>[2x]MKTDFIMVPTAMPDEKMINYQLAIDGGEPVIPKANRKTIFPNIAKEDLFQMMISVQKPEEMVVSEFAEKYRQRVGAPYAIPTASGTSSLHLALVGAGVKAGDEVIVPAFTFIATAQAIVAAKAIPVFADIDPQTYCLDPRQLDKKVTARTKAVMPVHVHGLPADIDALASFCRQHQLALIEDASHAHSATLHGRYCGTFGDAAGQSLMADKNFPLGGEAGIAFFKERESYDRALAFLEESGLDYRMSWVAAAFGISQLDRLDYYDEIRQRNAQRLIDELATTRLFTGPMI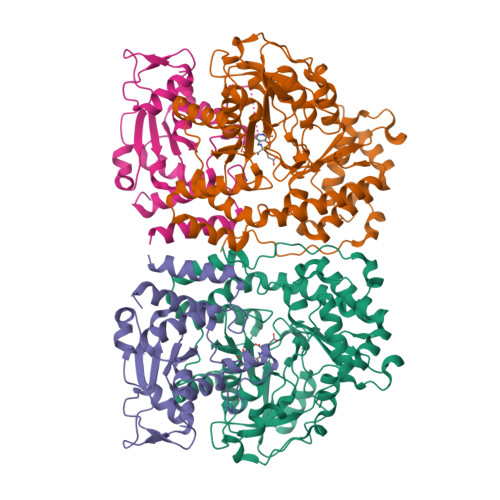PAAAKHSFNMFRIKINTALPEFKDIPEYKLKLALQQILNEEGVFAREWQNTLLPFHLPFQNKKGFGKGYPFFLGDSQEYKHEHFPNALQMLRSTLVLCRELRSPVEYEKLHSYIITFKKVDKNIQRVAEIASQIDDVPPYEKDARLGHHHHHH;>[2x]MGISKTSSDLSEQLFQVSFVLARVLTSGIIMSIEKNENELKGLENILKKTSSKQYAVTFNSISGAVIGSLWGQDIVYGEATNQQSLDEQQEKLFKWLGIGHSSLLPEPYTLHAINWGNISNLQKITHEEAHVTLLDFTKLGFGPCAVLLTNNETIYKKSERLKIFGAFDLRTMWTQRETEKEIKPGLQFNFRLSPLVGACIKMALIKMGLNKHHHHHH> GGAGAGUAGAUGAUUCGCGUUAAGUGUG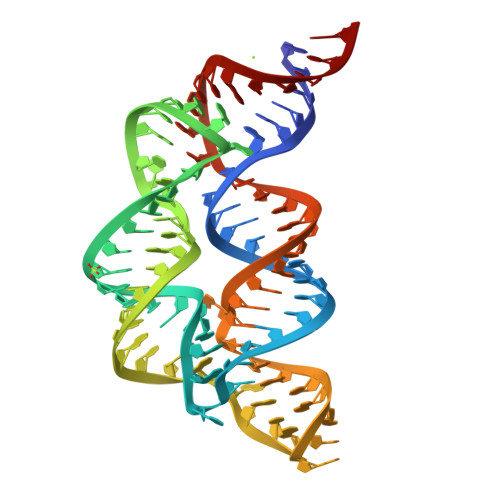UGUGAAUGGGAUGUCGUCACACAACGAAGCGAGAGCGCGGUGAAUCAUUGCAUCCGCUCCA>AGFMEAFLLENRKPKITTLASGKTLKPATHRLNLPAYTKLIHELRTKTHAKVTISLSTESQIHMVWVKSGLVFFTPSASHPAYVNFASSSRLTDVPALTKPTFPQSDAKLIESTPLPNDEASHVASFQLVTWKDGALSILNDLSKCAISFINQCEDTFKSGTNLNKEMYNRCITAESRDFCNQMKFVLIGRLCYGQTTSPPPIQLYQYG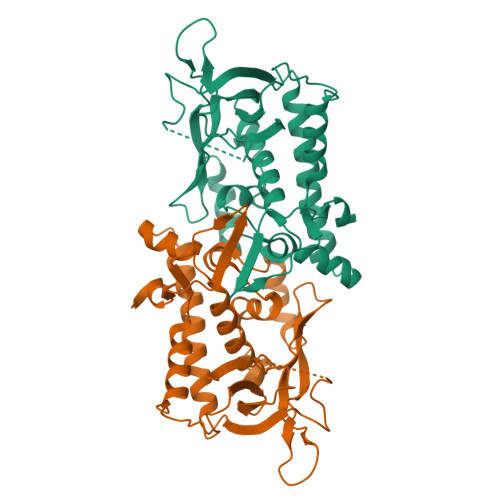VTPFISADIICEGAAYRSIDVENYAMNSNHLVSYAPFFVPNDTKPGSRIDLLMVNHLKKFNLIFDTWYKTGGSVMVSSRP[4x]> GKWVIDPSELTFVQEIGSGQFGLVHLGYWLNKDKVAIKTIREGAMSEEDFIEEAEVMMKLSHPKLVQLYGVCLEQAPICLVTEFMEHGCLSDYLRTQRGLFAAETLLGMCLDV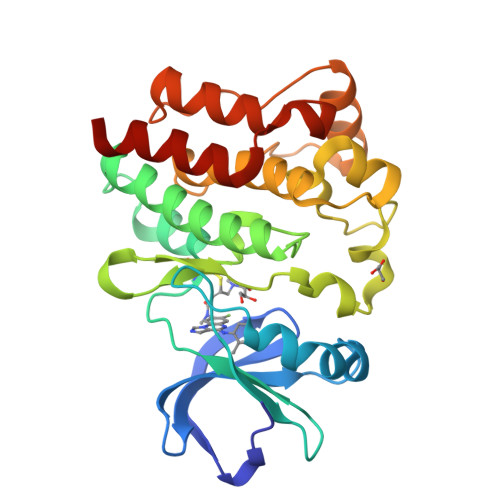CEGMAYLEEACVIHRDLAARNCLVGENQVIKVSDFGMTRFVLDDQYTSSTGTKFPVKWASPEVFSFSRYSSKSDVWSFGVLMWEVFSEGKIPYENRSNSEVVEDISTGFRLYKPRLASTHVYQIMNHCWRERPEDRPAFSRLLRQLAEIAESGL>ARSTNTFNYATYHTLDEIYDFMDLLVAQHPELVSKLQIGRSYEGRPIYVLKFSTGGSNRPAIWIDLGIHSREWITQATGVWFAKKFTENYGQNPSFTAILDSMDIFLEIVTNPNGFAFTHSENRLWRKTRSVTSSSLCVGVDANRNWDAGFGKAGASSSPCSETYHGKYANSEVEVKSIVDFVKNHGNFKAFLSIHSYSQLLLYPYGYTTQSIPDKTELNQVAKSAVAALKSLYGTSYKYGSIITTIYQASGGSIDWSYNQGIKYSFTFELRDTGRYGFLLPASQIIPTAQETWLGVLTIMEHTVNN[2x];>[2x]ZZHADPICNKPCKTHDDCSGAWFCQAC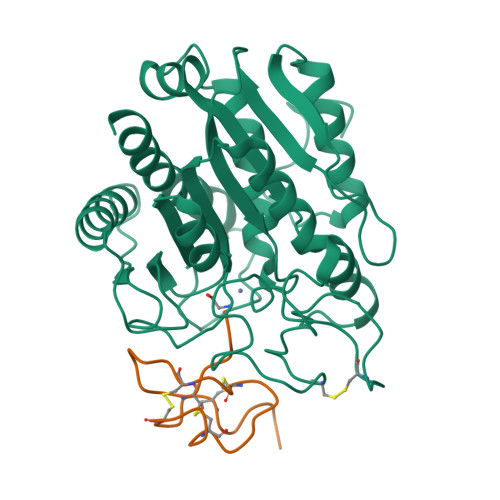WNSARTCGPYV>[5x]SQQFRIDS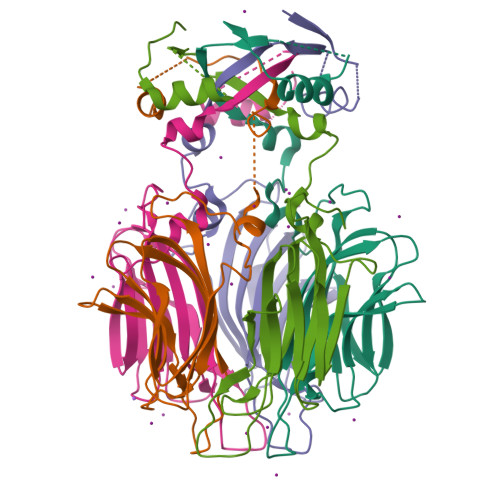ESIRDKLNTLLPSQSRGSIGVDLSGSTTIIPVVDLTETAEGGAQREDLQKAFTLINTIDFDVENTTTTIANTPGFYKVVGNLSSRDEASGAIAVIEVTDGITTKILANNRIVSPDGTTAVQSVPVPFDLMVKLVAGDTLQARSNNAEVRVQGIARQIADVSGNLINP>IQVTQPSVVLASSHGVASFPCEYSPSHNTDEVRVTVLRQTNDQMTEVCATTFTEKNTVGFLDYPFCSGTFNESRVN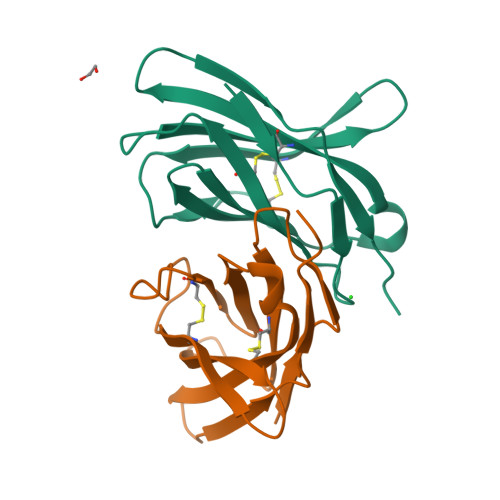LTIQGLRAVDTGLYLCKVELMYPPPYFVGMGNGTQIYVIDP[4x]>MAHHHHHHFRIVVGLGKSGMSLVRYLARRGLPFAVVDTRENPPELATLRAQYPQVEVRCGELDAEFLCSARELYVSPGLSLRTPALVQAAAKGVRISGDIDLFAREAKAPIVAITGSNAKSTVTTLVGEMAVAADKRVAVGGNLGTPALDLLADDIELYVLELSSFQLETCDRLNAEVATVLNVSEDHMDRYDGMADYHLAKHRIFRGARQVVVNRADALTRPLIADTVPCWSFGLNKPDFKAFGLIEEDGQKWLAFQFDKLLPVGELKIRGAHNYSNALAALALGHAVGLPFDAMLGALKAFSGLAHRCQWVRERQGVSY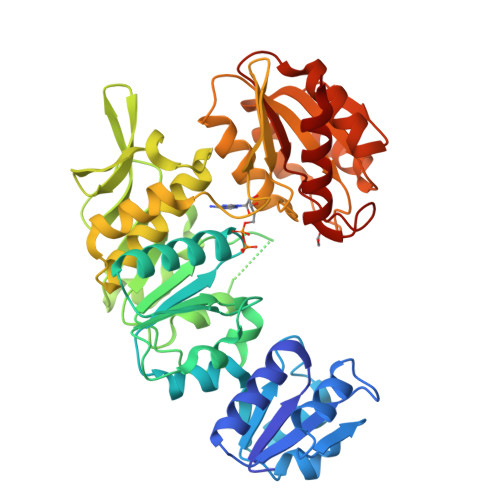YDDSKATNVGAALAAIEGLGADIDGKLVLLAGGDGKGADFHDLREPVARFCRAVVLLGRDAGLIAQALGNAVPLVRVATLDEAVRQAAELAREGDAVLLSPACASLDMFKNFEERGRLFAKAVEELA[3x]>[2x]SMIVKRGDVYFADLSPVVGSEQGGVRPVLVIQNDIGNRFSPTAIVAA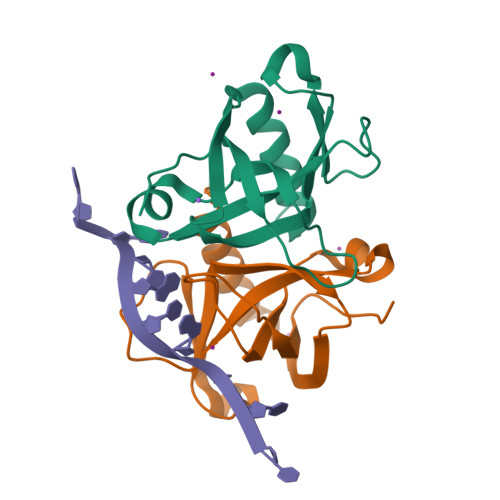ITAQIQKAKLPTHVEIDAKRYGFERDSVILLEQIRTIDKQRLTDKITHLDDEMMDKVDEALQISLALIDF>MSQKGKGSCPRPQQVPRLLVKGGIEVLDVKSGPDSITTIEAYLQPRPGQKNGYSTVITVQAEGYQDAPHSTEVPCYSCARIPLPTINDDITCPTLLMWEAVSVKTEVVGVSSILNMHSGAFRAFNGYGGGFTICGPRIHFFSVGGEP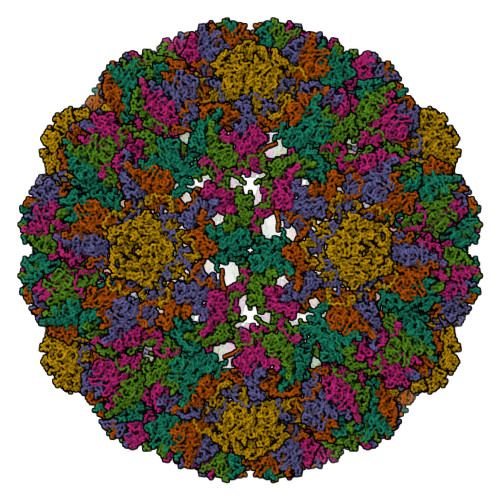LDLQACMQNSKTVYPAPLIGPGEGERRETAQVLDTGYKARLDKDGLYPIECWCPDPAKNENTRYYGNLTGGPETPPVLAFTNTTTTILLDENGVGPLCKGDGLFLSAADVAGTYVDQRGRQYWRGLPRYFSIQLRKRNVRNPYPVSGLLNSLFNDLMPRMTGQSMQGSDAQVEEVRVYEGMEGLAPEIDMPPKAPR[6x]> STTLTRQDLNFGQV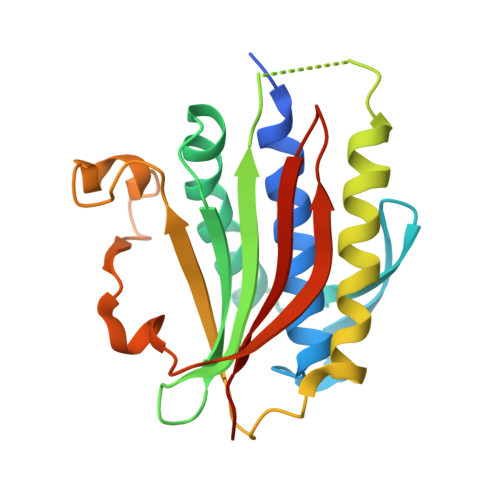VADVLCEFLEVAVHLILYVREVYPVGIFQKRKKYNVPVQMSCHPELNQYIQDTLHCVKPLLEKNDVEKVVVVILDKEHRPVEKFVFEITQPPLLSISSDSLLSHVEQLLAAFILKISVCDAVLDHNPPGCTFTVLVHTREAATRNMEKIQVIKDFPWILADEQDVHMHDPRLIPLKTMTSDILKMQLYVEERAHKGS> ASAKELACQEITVPLCKGIGYNYTYMPNQF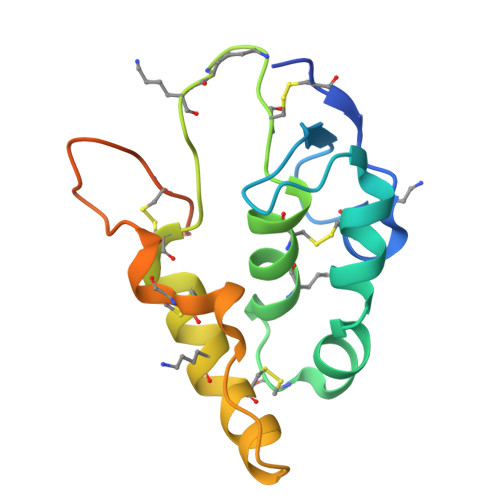NHDTQDEAGLEVHQFWPLVEIQCSPDLKFFLCSMYTPICLEDYKKPLPPCRSVCERAKAGCAPLMRQYGFAWPDRMRCDRLPEQGNPDTLCMDYNRTDLTTASRPAPELLG3-(4-methyl-3-oxo-3,4-dihydroquinoxalin-2-yl)propanoic acid 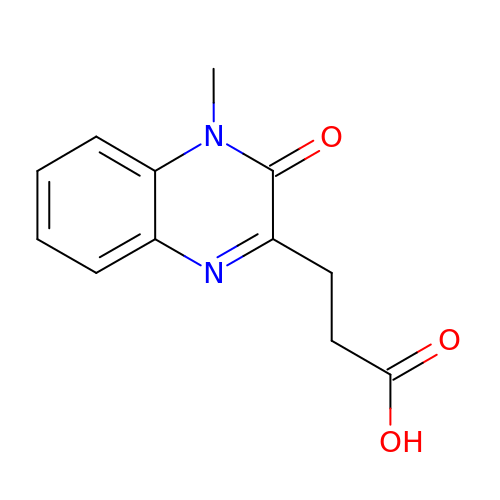| C12 H12 N2 O3 | JIXBAXULUJSRDR-UHFFFAOYSA-N> SATRANKDI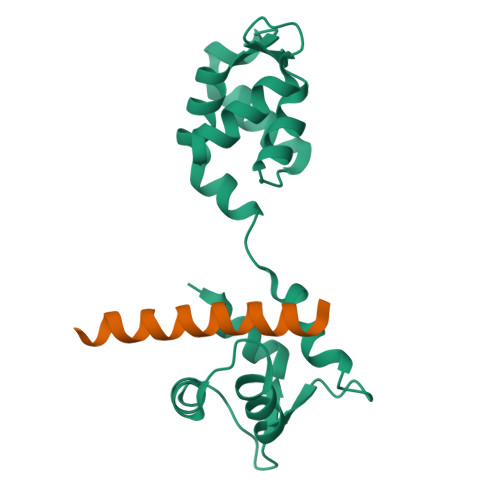FTLFDKKGQGAIAKDSLGDYLRAIGYNPTNQLVQDIINADSSLRDASSLTLDQITGLIEVNEKELDATTKAKTEDFVKAFQVFDKESTGKVSVGDLRYMLTGLGEKLTDAEVDELLKGVEVDSNGEIDYKKFIEDVLRQ;> SVLRTITNLQKKIRKELKQRQLKQE>[2x]GSMRTRVRARVISHALKDILAEGDKVIIMGHKRPDLDAIGAAIGVSRFAMMNNLEAYIVLNETDIDPTLRRVMNEIDKKPELRERFITSDDAWDMMTSK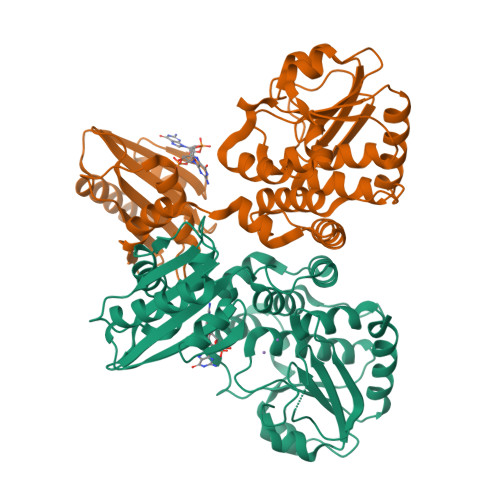TTVVIVDTHKPELVLDENVLNKANRKVVIDHHRRGESFISNPLLIYMEPYASSTAELVTELLEYQPTEQRLTRLESTVMYAGIIVDTRNFTLRTGSRTFDAASYLRAHGADTILTQHFLKDDVDTYINRSELIRTVKVEDNGIAIAHGSDDKIYHPVTVAQAADELLSLEGIEASYVVARREDNLIGISARSLGSVNVQLTMEALGGGGHLTNAATQLKGVTVEEAIAQLQQAITEQLSR>MDRKVQVLDFIKINPAGNITILIDNFDIYDKNIPKLSEEIMKETNLYAEQVGFIKDSHLQMMGGEFSGNASRAFASLLAFRDKDFSKQKNYNITCSGESKVLDVDVRNDGAKNKFLAKIKMPK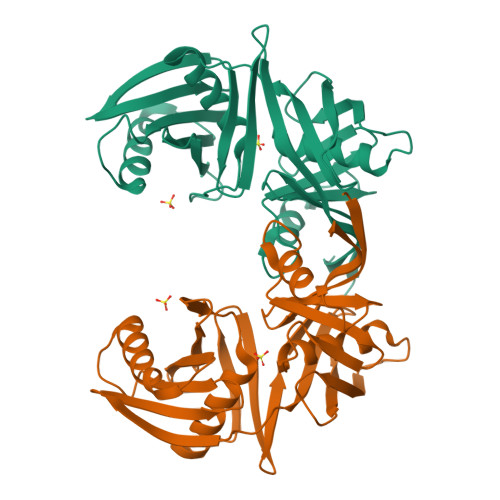FLSLEEINVDEYKLGLVRFSGINHFIFNIKENKETSFENIIDLVKKYLSNEEYSAFGIMFFDSDNLSMKPYVYVKEVGSGVYENSCASGTTALGYYLKKCKNLDRAKIVQPNGWLEYIIENDEMYIDGPVEIIAEGKIYIGKHHHHHH[4x]>[2x]GAMHSGIHVQHIKRRDIVLKRELGEGAFGKVFLAECYNLSPTKDKMLVAVKALKDPTLAARKDFQREAELLTNLQHEHIVKFYGVCGDGDPLIMVFEYMKHGDLNKFLRAHGPDAMILVDGQPRQAKGELGLSQMLHIASQIASGMVYL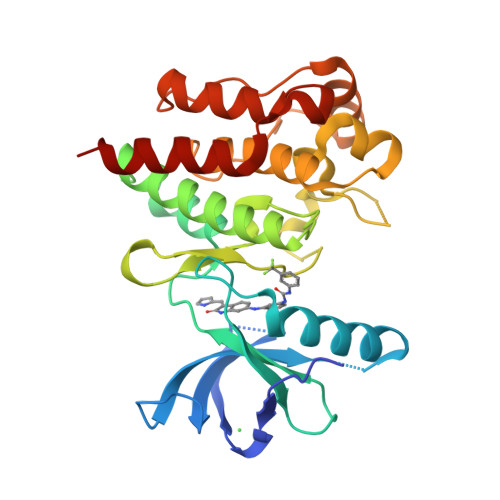ASQHFVHRDLATRNCLVGANLLVKIGDFGMSRDVYSTDYYRVGGHTMLPIRWMPPESIMYRKFTTESDVWSFGVILWEIFTYGKQPWFQLSNTEVIECITQGRVLERPRVCPKEVYDVMLGCWQREPQQRLNIKEIYKILHALGKATP> MEQPGLCGLSNLGNTCFMNSAIQCLSNTPPLTEYFLNDKYQEELNFDNPLGMRGEIAKSYAELIKQMWSGKFSYVTPRAFKTQVGRFAPQFSGYQQQDCQELLAFLLDGLHEDLNRIRKKPYIQLKDADGRPDKVVAEEAWENHLKRNDSIIVDIFHGLFKSTLVCPECAKISVTFDPFCYLTLPLASTSKVKLKDCIELFTTKEKLGAEDPWYCPNCKEHQQATKKLDLWSLPPVLVVHLKRFSYSRYMRDKLD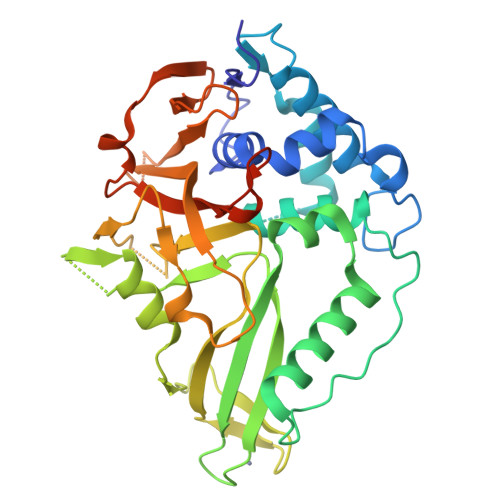TLVDFPINDLDMSEFLINPNAGPCRYNLIAVSNHYGGMGGGHYTAFAKNKDDGKWYYFDDSSVSTASEDQIVSKAAYVLFYQRQDTFSGTGFFPLDRETAAALEHHHHHH>MKAPVRVAVTGAAGQIGYSLLFRIAAGEMLGKDQPVILQLLGSERSFQALEGVVMELEDCAFPLLAGLEATDDPKVAFKDADYALLVGAAPRKAGMERRDLLQVNGKIFTEQGRALAEVAKKDVKVLVVGNPANTNALIAYKNAPGLNPRNFTA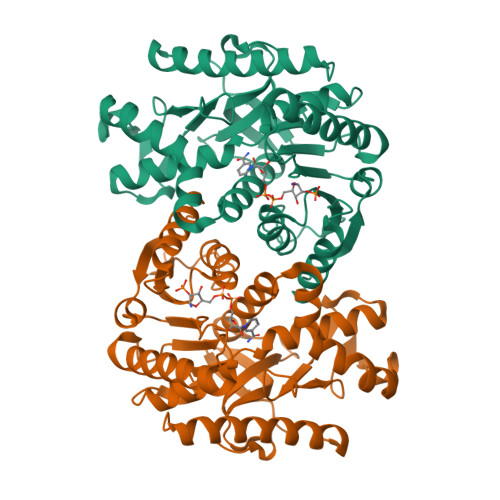MTRLDHNRAKAQLAKKTGTGVDRIRRMTVWGNHSSTMFPDLFHAEVDGRPALELVDMEWYEKVFIPTVAQRGAAIIQARGASSAASAANAAIEHIRDWALGTPEGDWVSMAVPSQGEYGIPEGIVYSFPVTAKDGAYRVVEGLEINEFARKRMEITAQELLDEMEQVKALGLI[2x]>ETQQRCVTATDYDTFVSERFGSIIQAVQTFTDSTKPGYAFIAAKPKSGLYLTTVQREDIKNYLKDYNLAPITPSIISPNYLFIKTNLKVTYALNKLQESEQWLEGQIIDKIDRYYTEDVEIFNSSFAKSKMLTYVDDADHSVIGSSATIQMVREVQNFYKTPEAGIKYNNQIKDRSMESNTFSFNSGRKVVNPDTGLEEDVLYDVRIVSTDRDSKGIGKVIIGPFASGDVTENENIQPYTGNDFNKLANSDGRDKYYVIGEINYPADVIYWNIAKINLTSEKFEVQTIELYSDPTDDVIFTR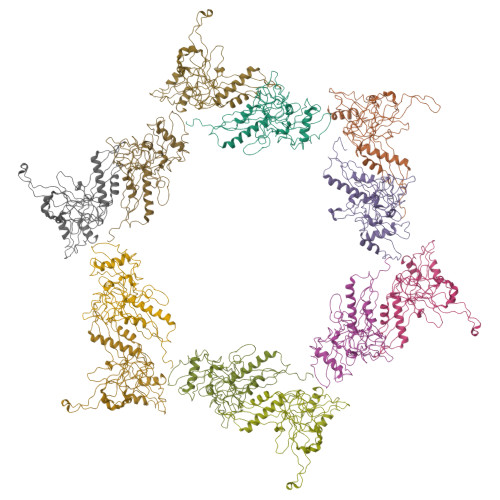DGSLIVFENDLRPQYLTIDLEPISQLEHHHHHH[12x]> AYVVTDNCIKCKYTDCV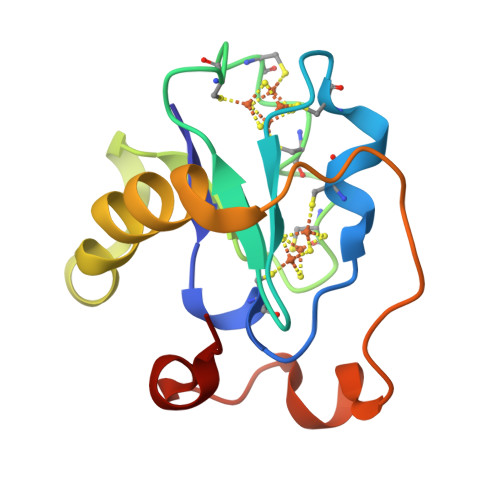EVCPVDCFYEGPNFLVIHPDECIDCALCEPECPAQAIFSEDEVPEDMQEFIQLNAELAEVWPNITEKKDPLPDAEDWDGVKGKLQHLER>[2x]GPGSMAFKLPALPYGMRELIPHISEETLSFHYGKHHAGYVNKLNSLIKGTPMESCTIEELILGQTGAVFNNAAQIWNHTFYWNSMGPNCGGEPTGPIRKKIEEK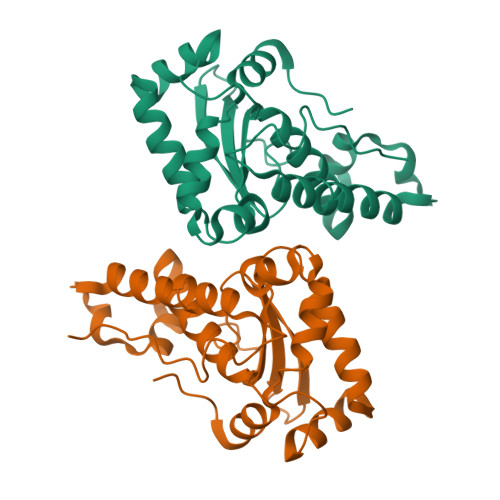FGSFSAFKTDFSNLLAGHFGSGWGWLVLKDDGTADIVQTHDAGSPLKENLGRPLLCCDVWEHAYYIDYKNDRLSYINSWWNLVNWDFANKNLEAPFKWS>MEIPVIEPLFTKVTEDIPGATGPVFDKNGDFYIVASPLSEALTKANSPAEAYKASRGAGEILRIDLKTGKKTVICKPEVNGYGGSPIGCQCDRDANQLFVADMRLGLLVVQTDGTFEEIAKKDSEGRRMQGCAYCAFDYEGNLWITAPAGEVAPADFTISLREKFGSIYCFTTDGQMIQVDTAFQCPAGIAVRHMNDGRPYQL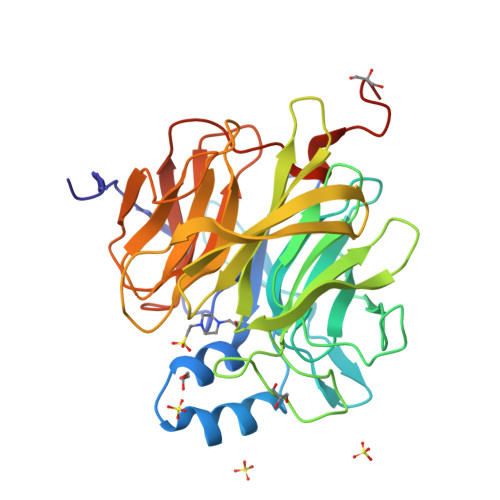IVAEQPTKKLWSYDIKGPAKIENKKVWGHIPGTHKGGAAGMDFDEDNNLLVANWGSSHIEVFGPDGGQPKMRIRCPFEKPANLHFKPQTKTIFVTEHENNAVWKFEWQRNGKKQYCETLKFGIFGSLEHHHHHH[2x]>[2x]METYTVKLGSDK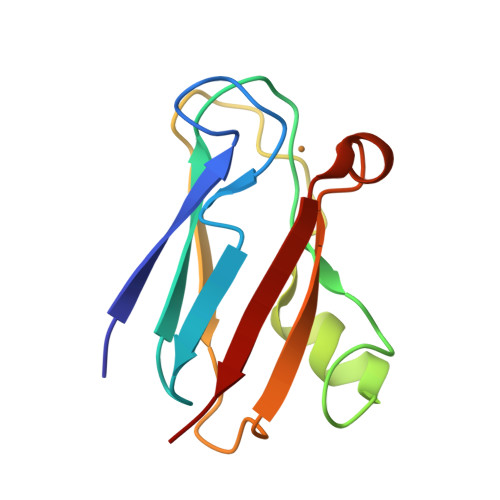GLLVFEPAKLTIKPGDTVEFLNNKVPPHNVVFDAALNPAKSADLAKSLSHKQLLMSPGQSTSTTFPADAPAGEYTFYCEPHRGAGMVGKITVAG propane-1,1,1,3-tetrol | C3 H8 O4 | 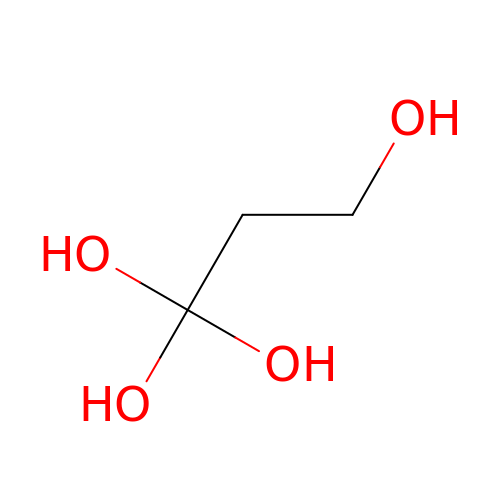VQAQNRIKRHUZBR-UHFFFAOYSA-N> MGDLSCPEGLEELLSAPPPDLGAQRRHGWNPKDCSENIEVKEGGLYFERRPVAQSTDGARGKRGYSRGLHAWEISWPLEQRGTHAVVGVATALAPLQTDHYAALLGSNSESWGWDIGRGKLYHQSKGPGAPQYPAGTQGEQLEVPERLLVVLDMEEGTLGYAIGGTYLG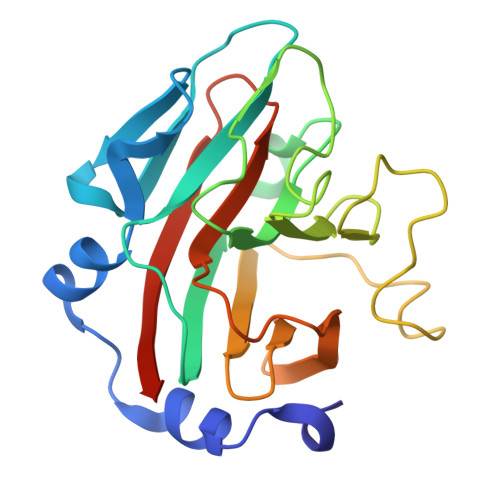PAFRGLKGRTLYPAVSAVWGQCQVRIRYLGERGSHHHHHH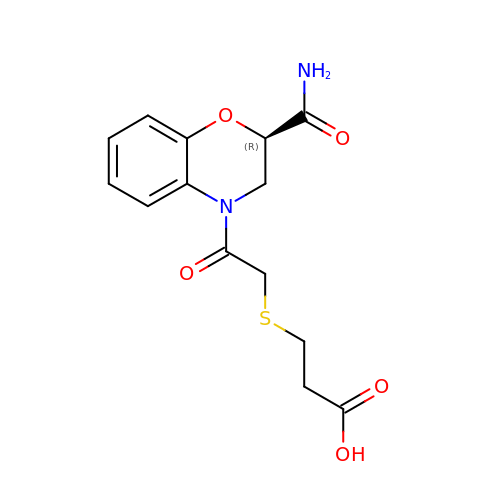3-({2-[(2R)-2-carbamoyl-2,3-dihydro-4H-1,4-benzoxazin-4-yl]-2-oxoethyl}sulfanyl)propanoic acid | C14 H16 N2 O5 S | SDNYVGUVTOZEQL-LLVKDONJSA-N The core particle of the proteasome (20S CP) associates with ring-shaped activator complexes to degrade protein substrates. Alternatively, the 20S CP can associate with the bacterial proteasome activator (Bpa) and degrade proteins in a pupylation-independent manner. Bpa monomers feature a four-helix bundle fold and assemble into a dodecameric, ring-shaped complex with the protomers arranged around a large central opening of about 40 Å in diameter. Unlike Mpa, Bpa facilitates the proteasomal degradation of its substrates without making use of a tagging system like pupylation and without the expense of ATP.

While high-resolution structures of truncated Bpa have been determined previously using X-ray crystallography, the conformation of the full-length Bpa dodecamer in its unbound state has not been addressed. To confirm that full-length Bpa in its unbound state behaves similarly to the previously studied truncated Bpa constructs, we determined its structure using cryo-EM. The cryo-EM map of full-length Bpa was resolved at 3.2 Å with local resolution ranging from 2.7 to 3.4 Å. Similar to the crystal structures published previously, our model confirmed that the Bpa protomer forms a tight four-helix bundle. However, in contrast to existing models, our structure showed that the helical extensions of helix H4 exhibit greater flexibility. It appears that the crystal packing in the X-ray crystallography structure of truncated Bpa (residues 15-153), resulted in stabilization of helix H4 up to residue L14821. Our cryo-EM maps showed no discernable density beyond Bpa residue Q140 within the H4 extension, indicating that the residues following Q140, while possessing helical propensity, are dynamic. At the N-terminal side, the first Bpa residue that could be resolved confidently was S36 which is located toward the same ring face of Bpa as the C-terminal H4 extension. This demonstrates that the first 35 residues are disordered and emanate from the Bpa face oriented toward the CP α-ring in the Bpa-CP complex. Comparing this structure to the structure of full-length Bpa determined in the absence of substrate, we could not identify significant differences within the dodecameric Bpa ring itself.

>[12x]MHHHHHHMVIGLSTGSDDDDVEVIGGVDPRLIAVQENDSDESSLTDLVEQPAKVMRIGTMIKQLLEEVRAAPLDEASRNRLRDIHATSIRELEDGLAPELREELDRLTLPFNEDAVPSDAELRIAQAQLVGWLEGLFHGIQTALFAQQMAARAQLQQMRQGALPPGVGKSGQHGHGTGQYL>[4x]ATAVNGAPRDAALWSSHEQMLAQPLKDSDAEVYDIIKKESNRQRVGLELIASENFASRAVLEALGSCLNNKYSEGYPGQRYYGGTEHIDELETLCQKRALQAY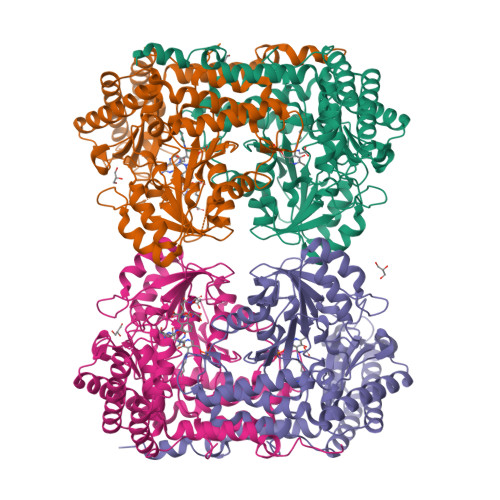GLDPQCWGVNVQPYSGSPANFAVYTALVEPHGRIMGLDLPDGGHLTHGFMTDKKKISATSIFFESMAYKVNPDTGYIDYDRLEENARLFHPKLIIAGTSCYSRNLDYGRLRKIADENGAYLMADMAHISGLVVAGVVPSPFEHCHVVTTTTHKTLRGCRAGMIFYRRGVRSVDPKTGKEILYNLESLINSAVFPGLQGGPHNHAIAGVAVALKQAMTPEFKEYQRQVVANCRALSAALVELGYKIVTGGSDNHLILVDLRSKGTDGGRAEKVLEACSIACNKNTCPGDKSALRPSGLRLGTPALTSRGLLEKDFQKVAHFIHRGIELTVQIQDDTGPRATLKEFKEKLAGDEKHQRAVRALRQEVESFAALFPLPGLPGF>[6x]MASMTGGQQMGRGSMSILDIAGVDDTLQRLLKEVWFPLRGGEACEKMGYRYDNGVLLHGPSGCGKTTLAHAIAGSIGVAFIPVSAPSVIGGTSGESEKNIRDVFDEAIRLAPCLIFLDQIDAIAGRRESANKGMESRIVAEIMNGMDRIRQNTPLGKNVVVLAATNRPEFLDPAIRRRFSVEIDMGMPSERAREQILRSLTRDLSLADDINFKELAKMTPGYVGSDLQYVVKAAVSESFQANIDSLLAQARAKHPADHLANVSQPQRDWLLLEAHRDEEVSWPSTKITMEQFRKAVSLVQPASKREGFSTIPDTTWSHVGALEDVRKKLEMSIIGPIKNPELFTRVGIKPAAGILLWGPPGCGKTLVAKAVANESKANFISIKGPELLNKYVGESERAVRQLFSRAKSSAPCILFFDQMDALVPRRDDSLSDASARVVNTLLTELDGVGDRSGIYVIGATNRPDMIDEAIRRPGRLGTSIY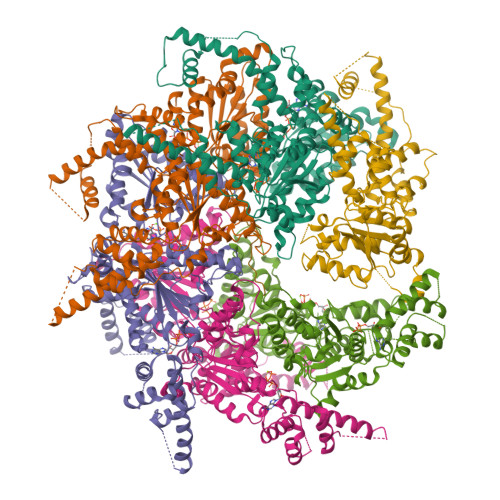VGLPSAEDRVKILKTLYRNTVKAPKKREGTNGEDVDMTDAAAEQQHQGTTDADLEKVALDLRCTGFSGADLGNLMQAAAQACLERVYTQRQQKRKEGGSVAEEEEIEPVITMEDWEKALNEVKPSVKDPEKYMHSGFAAALEHHHHHH;> LLLLLLLLLLLLLLLLLLLLLLLL> HMKWTPPRSPFNLVQEILFHDPWKLLIATIFLNRTSG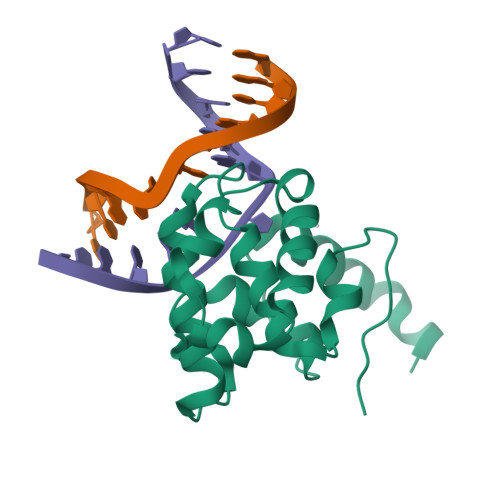KMAIPVLWEFLEKYPSAEVARAADWRDVSELLKPLGLYDLRAKTIIKFSDEYLTKQWRYPIELHGIGKYGNDSYRIFCVNEWKQVHPEDHKLNKYHDWLWENHEKLSLS>MTRILTAFKVVRTLKTGFGFTNVTAHQKWKFSRPGIRLLSVKAQTAHIVLEDGTKMKGYSFGHPSSVAGEVVFNTGLGGYPEAITDPAYKGQILTMANPIIGNGGAPDTTALDELGLSKYLESNGIKVSGLLVLDYSKDYNHWLATKSLGQWLQEEKVPAIYGVDTRMLTKIIRDKGTMLGKIEFEGQPVDFVDPNKQNLIAEVSTKDVKVYGKGNPTKVVAVDCGIKNNVIRLLVKRGAEVHLVPWNHDFTKMEYDGILIAGGPGNPALAEPLIQNVRKILESDRKEPLFGISTGNLITGLAAGAKTYKMSMANRGQNQPVLNITNKQAFITAQNHGYALDNTLPAGWKPLFVNVNDQTNEGIMHESKPFFAVQFHPEVTPGPIDTEYLFDSFFSLIKKGKATTITSVLPKPALVASRVEVSKVLILGSGGLSIGQAGEFDYSGSQAVKAMKEENVKTVLMNPNIASVQTNEVGLKQADTVYFLPITPQFVTEVIKAEQPDGLILGMGGQTALNCGVELFKRGVLKEYGVKVLGTSVESIMATEDRQLFSDKLNEINEKIAPSFAVESIEDALKAADTIGYPVMIRSAYALGGLGSGICPNRETLMDLSTKAFAMTNQILVEKS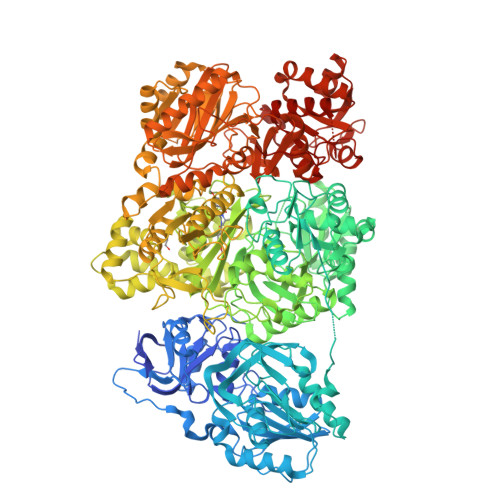VTGWKEIEYEVVRDADDNCVTVCNMENVDAMGVHTGDSVVVAPAQTLSNAEFQMLRRTSINVVRHLGIVGECNIQFALHPTSMEYCIIEVNARLSRSSALASKATGYPLAFIAAKIALGIPLPEIKNVVSGKTSACFEPSLDYMVTKIPRWDLDRFHGTSSRIGSSMKSVGEVMAIGRTFEESFQKALRMCHPSIEGFTPRLPMNKEWPSNLDLRKELSEPSSTRIYAIAKAIDDNMSLDEIEKLTYIDKWFLYKMRDILNMEKTLKGLNSESMTEETLKRAKEIGFSDKQISKCLGLTEAQTRELRLKKNIHPWVKQIDTLAAEYPSVTNYLYVTYNGQEHDVNFDDHGMMVLGCGPYHIGSSVEFDWCAVSSIRTLRQLGKKTVVVNCNPETVSTDFDECDKLYFEELSLERILDIYHQEACGGCIISVGGQIPNNLAVPLYKNGVKIMGTSPLQIDRAEDRSIFSAVLDELKVAQAPWKAVNTLNEALEFAKSVDYPCLLRPSYVLSGSAMNVVFSEDEMKKFLEEATRVSQEHPVVLTKFVEGAREVEMDAVGKDGRVISHAISEHVEDAGVHSGDATLMLPTQTISQGAIEKVKDATRKIAKAFAISGPFNVQFLVKGNDVLVIECNLRASRSFPFVSKTLGVDFIDVATKVMIGENVDEKHLPTLDHPIIPADYVAIKAPMFSWPRLRDADPILRCEMASTGEVACFGEGIHTAFLKAMLSTGFKIPQKGILIGIQQSFRPRFLGVAEQLHNEGFKLFATEATSDWLNANNVPATPVAWPSQEGQNPSLSSIRKLIRDGSIDLVINLPNNNTKFVHDNYVIRRTAVDSGIPLLTNFQVTKLFAEAVQKSRKVDSKSLFHYRQYSAGKAA[2x]>[2x]MAPNNTQQEEASKGGNSSPEAYLPYSGDIAIAGISGRYPESDSVGEFRDNLFGKVNMLTCDDRRWKLGHLDLPDVLGKLRSVDRFDSEFFNLNSKQTEMLDPQTRLLLEVCYEAIVDAGESLASVKGSRTGMYLAISSSEPEQAWICRQDPYIVMGCPHTMSPNRISFFFDLHGPSIAYDTACSSVLVALEAAFQHMRTGVIDSAIVAGVNTCFRALTSKVYQNMGMLGPEACKAFDSSGNGYARSEIVSALFLKKSSDSKRIYCSVVNVKTNNDGFTPQGLTFPSGEIQEQLMRNVYADCKLNPKEVSYFECHGTGTPAGDPQETNAIYRVMCTPDKREPLLIGSVKSNMGHAETGSAMASITKVILAMHEGFIAPNLHFRSPNPKIEGLRDGKMAVVTEATPWSGGYMAINSFGMGGSNAHAVLRSYDVSSSKPHPSAHKPRLFTYSARTEHGLRAILREAQTHAASMEFHALCQASADAPLGSMPYRGATILNGQHDFEVVEKCKSKAREVWFIYAGMGSQWVGMARCLMQLDVFRHSLEKSAAVLKPHGVDLLNILSEGTEDTLRTILNPFVCITSIQVALTDLLWSMGIRPDGIVGHSMGEVGCAYCDGCLTAEEAVLTAYWRGKCVTDGKVPPGKMAAVGLTWEEAKSQCPAGVVPACHNAEDSVTISGAADVMLKFMEELKAKDVFVREVNSSNIAYHSYFMENIYASLKDSLSKVISPKPRTARWLPTSVPEELWDSAPAQSSSAEFHANNLVSPVLFHEALQKIPPTAIAIELAPHGLLQSVIKRTLGNESVCVGLQKRNYADNLEFLFASLGKCFANGLSLNPLACYPPVEFPVPKGTPRLSDMVAGAWDHSAQWLVPKNEDFEGRVQASGSDSSYSIDVSADSPDRYLLDHQVDGRELFPACGCLVLAWKTLAALNGRDFEQMPVRLSRVEIHQAMFLPKSGSATVTVSVMPRTGEFQVCENENLLASGFVTCPDKDVLETSTHAQTRSSLQDRPATEVLTRDEVYRELILRGYEYGPYFQGILRASVDGQESEITWDGRWVSFMDSVLQMDILARPGDYQMLPIKFQSINIDPRVQPAAPAEDEDVVVLPGRFDPVLDIVSAGGVEIRGLETISASRRLTHAPEVVEEYRFVPHHVTGRDDPGAKRPGATVDIREYADACLAFAVQGIKKWLSEDKDKVLPQKDLLQDALGLANQDLGSKSSSSDFISAKAALERILKQQNGHQQHGFGLFHTLNLAFSEPLEIGFRETLKNKIHHMRYDMWDDCLMSAVECADSLKLCIDTVAENTTSHIVNVLEAGAAKGAFYRRAIPEALAKFSGKDYRYTVGDASPMDDAKEFSVKTLQFDAYDPANFPASQAHAHDLLVLKWVLHQQEDLDAAMAGFCGFVRPGGFILVQEFVHRLPTLLAVEAVTDHPLPRKSGDRVLGRYYSAAQWRELFRRHGLVEVIHRSDGALADMFLLRSRVEVMTPPTVLHLDDLSCSWLEEVKAKYSDLEAMPQDARLWLVGKSDCNGMLGFFNCLRQEPGSERVRCVQVCGDSVPDLSPGSAEFKYLAEMDLAFNVHKDGKWGVYRHLAITDDQRRQQFPTEHAFVDTL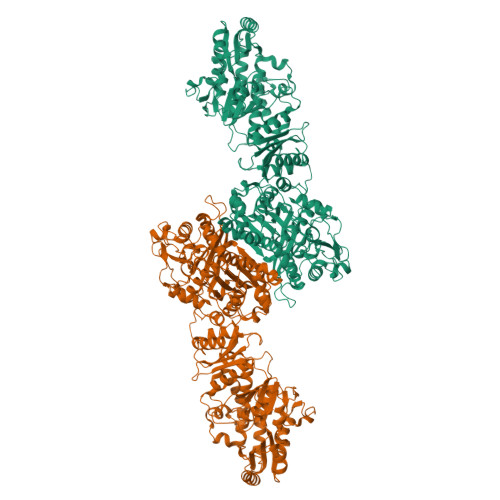TSGDLSTLTWVRSPLNLHASSEKGQDCELCTVYMAGVVSRDLALACGKLRRDELPAGMFCKEGTLGIEFSGRDTKGKRVMGLCAPPALASSVLCLRSSLWSVPQHWSLEEAATVPVAYSTAYYALVIRGHVRPGDTVLVHAGGSPVGQAAIAVAQSCGCEIFISTATDAETSSLKSMFPRLKDRNFCSCKDASFERHVKKETSGKGVDIILNCTTGELLGASIRLLASRGRFLNLASGRGSDAELVFSGSGRRDTSFHDINLDTLIDAQGPEWTELTSLVQKGIQSGLVKPLARTVYAMDRLVDVFKLLEEGAQAGKLLVKIREEEAEKITLPAKKTFEAVPRTFFHPAKSYVIVGGLGGFGLELAHWMVLRGVRKLVLTSRNGITTGYQTRKIAFLRSLGADIVVCAVNVTSQAAADRLVKTATDLGPLGGVFNLGLNLRDALLVEQTAENYKQTLEAKIQTTSLLDGISRSPKIQPTLDHFVMFSSLSAGHGIPGQTNYGWGNSYMDRLCEKRRAQGLPGLSIQWASIADVGFVGTKGNNVVIEGKWPQRMYNCLQVCDYFLSQNRPVVACHVLAEKVKAAVEGEETVGQQVIKAVGNVLGLKSVSGVDPDKVFLDLGLDSLMSVEIKQMLERDLDLALGTKDIQMLTFAQLQAMVQHVHHHHHH>MWFGEFGGQYVPETLIEPLKELEKAYKRFKDDEEFNRQLNYYLKTWAGRPTPLYYAKRLTEKIGGAKIYLKREDLVHGGAHKTNNAIGQALLAKFMGKTRLIAETGAGQHGVATAM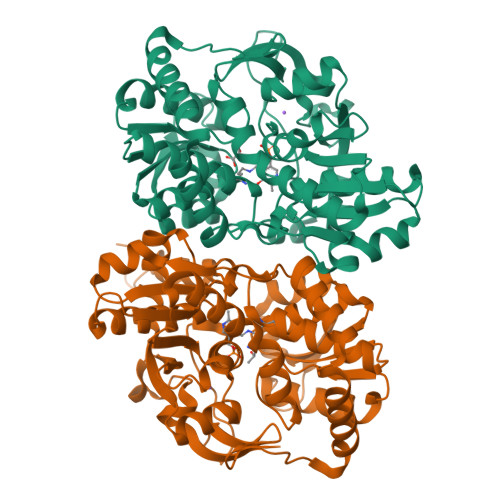AGALLGMKVDIYMGAEDVERQKMNVFRMKLLGANVIPVNSGSRTLKDAINEALRDWVATFEYTHYLIGSVVGPHPYPTIVRDFQSVIGREAKAQILEAEGQLPDVIVACVGGGSNAMGIFYPFVNDKKVKLVGVEAGGKGLESGKHSASLNAGQVGVFHGMLSYFLQDEEGQIKPTHSIAPGLDYPGVGPEHAYLKKIQRAEYVTVTDEEALKAFHELSRTEGIIPALESAHAVAYAMKLAKEMSRDEIIIVNLSGRGDKDLDIVLKVSGNVLEHHHHHH[4x]>LQMIDVHQLKKSFGSLEVLKGINVHIREGEVVVVIGPSGSGKSTFLRCLNLLEDFDEGEIIIDGINLKAKDTNLNKVREEVGMVFQRFNLFPHMTVLNNITLAPMKVRKWPREKAEAKAMELLDKVGLKDKAHAYPDSLSGGQAQRVAIARALAMEPKIMLFDEPTSALDPEMVGEVLSVMKQLANEGMT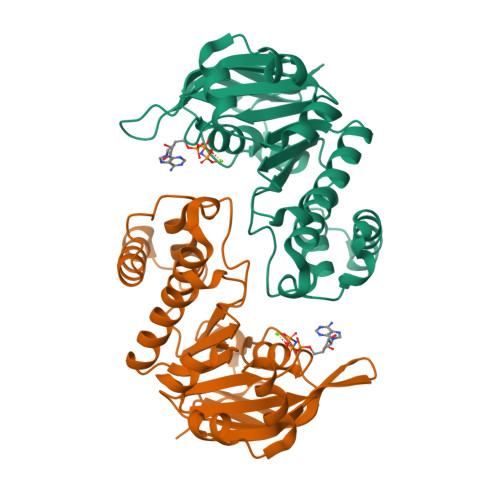MVVVTHEMGFAREVGDRVLFMDGGYIIEEGKPEDLFDRPQHERTKAFLSKVF[2x]We have described herein the reactions and the structure of Pgp3, a Csd protein of C. jejuni. This enzyme turns over the cell-wall peptidoglycan by both the d,d-endopeptidase and d,d-carboxypeptidase activities, as documented by mass spectrometric characterization of the requisite reactions with synthetic cell-wall fragments. The Pgp3 monomer is structurally divided into four regions: the N-terminal domain (NTD, residues 21–95), a flexible linker (residues 96–147), the LytM domain (residues 148–259), and the C-terminal helix (residues 260–273). The Pgp3 LytM domain contains a highly conserved tetrahedral Zn2+-ion-binding motif (H168xxxD172 and HxH249).

By using the H247A mutant variant, we successfully solved two structures of Pgp3 in complex with a pentapeptide (1, Ac-l-Ala1-γ-d-Glu2-mDAP3-d-Ala4−d-Ala5) and with a crosslinked muramyl tetra-tri peptide (2, NAM-l-Ala1-γ-d-Glu2-mDAP3-d-Ala4−mDAP3-γ-d-Glu2-l-Ala1-NAM). In the presence of the pentapeptide, excellent electron-density map was obtained for the mDAP3-d-Ala4-d-Ala5 segment. The importance of these two complexes is that the scissile bond in the peptide substrate was seen bound within the active site. The critical portions of both peptides with Pgp3 are shared motifs between the two structures. Both peptides contain the common motif, mDAP3-d-Ala4, and only the third amino acid is different, i.e., mDAP3 vs Ala5. In the pentapeptide-bound complex, Arg158 might form salt-bridge interactions with d-Ala5. Substrate carbonyl oxygen displaces Wat-2, thereby interacting directly with Zn2+ and polarizing the d-Ala4 carbonyl bond. This renders the amide bond susceptible to nucleophilic attack by Wat-1.

> MELIKGQALFLELDKKDFLSLKNNDKNIPTFAHPKNQEKILAIFSLPYKNPPQNTKLIAFYKDKKEEIFIKTLEGNYKSEKLQVENKKIFPPKTIQERIAKELKEANAIYSSYTPKALFNGAFNIPLNSFITSDFGKARTFNEKVASYHSGTDFRAATGTPIYAANSGVVKIAKDRYFAGNSVVIDHGFGIYSQYYHLSKIDVKVGQKIKKGELIGLSGASGRVSGPALHFGILAGGKQVDPLDFVSKFNAIFQ>[2x]KEFTLDFSTAKTYVDSLNVIRSAIGTPLQTISSGGTSLLMIDSGTGDNLFAVDVRGIDPEEGRFNNLRLIVERNNLYVTGFVNRTNNVFYRFADFSHVTFPGTTAVTLSGDSSYTTLQRVAGISRTGMQINRHSLTTSYLDLMSHSGTSLTQSVARAMLRFVTVTAEALRFRQIQRGFRTTLDDLSGRSY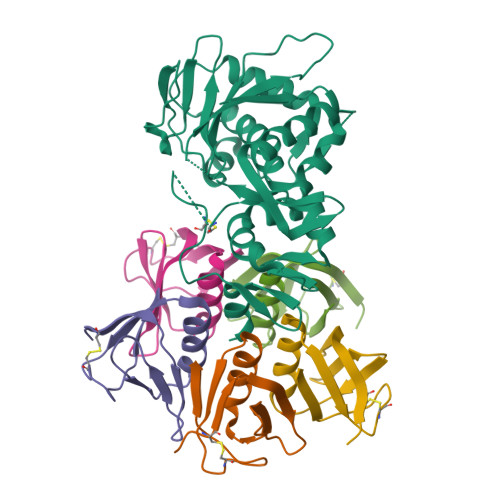VMTAEDVDLTLNWGRLSSVLPDYHGQDSVRVGRISFGSINAILGSVALILNCHHHASRVARMASDEFPSMCPADGRVRGITHNKILWDSSTLGAILM;>TPDCVTGKVEYTKYNDDDTFTVKVGDKELFTNRWNLQSLLLSAQITGMTVTIKTNACHNGGGFSEVIFR[10x]GEN1 is a member of the FEN/EXO family of structure-selective nucleases that cleave 1 nt 3′ to a variety of branchpoints. By contrast GEN1 cleaves DNA 1 nt 3′ to the point of strand exchange on two strands of four-way junctions, and the key distinction from the other members of the family is that it acts as a homodimer and thus makes two incisions into the junction. As we have found previously, the structure of CtGEN1 contains a central seven-strand β-sheet flanked on both sides by 15 α-helices, with a topology very similar to the other FEN/EXO family of nucleases. For each, the H2TH motif binds a monovalent ion and plays an important role in binding one helical arm of the substrates.

Wild-type CtGEN1 bound to a four-way junction was crystallized in the presence of Na+ and Mg2+ ions, resulting in crystals of a product complex because under these conditions CtGEN1 is active. These crystals were then soaked in either K+ or Cs+ ions to replace the Na+ ions. While the overall structure of the CtGEN1 product complex following a crystal soak with K+ ions is closely similar to the Cs+-bound structure, the H2TH region between α-helices 9 and 10 takes a significantly different trajectory. The C-terminal end of the loop (I205 to G209) adopts the same conformation as that in the Cs+ structure (RMSD = 0.21 Å), so that the K+ ion is positioned similarly to Cs+, and the main chain O atoms of I205 and C208 together with S196 at the N-terminal end bind the K+ ion in the same manner. However, the main chain O of D203 is 8.7 Å from the K+ metal ion, and this is the major difference between the metal ion coordination in the two structures. The K+ ion is coordinated by the two non-bridging O atoms of the DNA phosphate in the same manner as the Cs+ ion. The N-terminal section of the loop between G196 and G204 takes a very different trajectory in the K+ structure. The effect of this is that the loop is less extended compared to the Cs+ structure, thus disrupting the interaction of D203 with the monovalent metal ion. Importantly, D199 is no longer within the active site in the K+ structure, and its carboxylate is 12 Å from the M2 Mg2+ ion. In Na+ and K+ ions the loop is less extended, so that the D199, Y200 is substantially retracted away from the active site. First, the K+ and Cs+ crystals were generated by soaking the Na+-bound CtGEN1 crystals, rather than being crystallized in the presence of the respective monovalent ions.

> MGIKGIYKEIGSGERISLCKLAIDHLEQHNRPLRLAIDMAIWQFQIQAARGGSNPAIRTLFYRFVRLLSLGIHPIFVFDGPNKPIFKRNRRSGTGNGVSTAMAKRLIRLFGFTAHDAPGEAEAECAYLEQQGIVDAVLSEDVDTIMFGSRVTLRDWSSEGSKGGPPTHVTLHDAKKIAEGPSGLDREGMVLVALMSGGDYLPDGIPGCGIKVACQAAKAGFGKELCRIKRADKEAITEWKQRLLHELRTNESGFFRTKHKALEIPENFPNMEVLRYYTHPVVSSPATIERLRQEFPPSSTVDIAGLREFTRETFDWTFRPGAIKLIKVLAPGLLVQRCLDRYVSGPRIDDPDLKKKEESTLVKGISMRREHFSTDATPELRVSFIPAELVGLDPGQEPEVQVEAFGRSGLALNSDDEFDEDISSSQKAPKKPFDPWQPDLAWVPETILKLGVPVTVEDWEEGQRSKGRAKEDKTAAKAKRKTKIIQSNMPAGALDKYVTVTKNISDTTVKSKESAPITIPSSPPKPSSQP>SSGLNDIFEAQKIEWHEGSAGGSGGSGRSSLDNIEMAYARQIYIYNEKIVNGHLQPNLVDLCASVAELDDKSISDMWTMVKQMTDVLLTPATDALKNRSSVEVRMEFVRQALAYLEQSYKNYTLVTVFGNLHQAQLGGVPGTYQLVRSFLNIKLPAPLPGLQDGEVEGHPVWALIYYCMRCGDLLAASQVVNRAQHQLGEFKTWFQEYMNSKDRRLSPATENKLRLHYRRALRNNTDPYKRAVYCIIGRCDVTDNQSEVADKTEDYLWLKLNQVCFDDDGTSSPQDRLTLSQFQKQLLEDYGESHFTVNQQPFLYFQVLFLTAQFEAAVAFLFRMERLRCHAVHVALVLFELKLLLKSSGQSAQLLSHEPGDPPCLRRLNFVRLLMLYTRKFESTDPREALQYFYFLRDEKDSQGENMFLRCVSELVIESREFDMILGKLENDGSRKPGVIDKFTSDTKPIINKVASVAENKGLFEEAAKLYDLAKNADKVLELMNKLLSPVVPQISAPQSNKERLKNMALSIAERYRAQGISANKFVDSTFYLLLDLITFFDEYHSGHIDRAFDIIERLKLVPLNQESVEERVAAFRNFS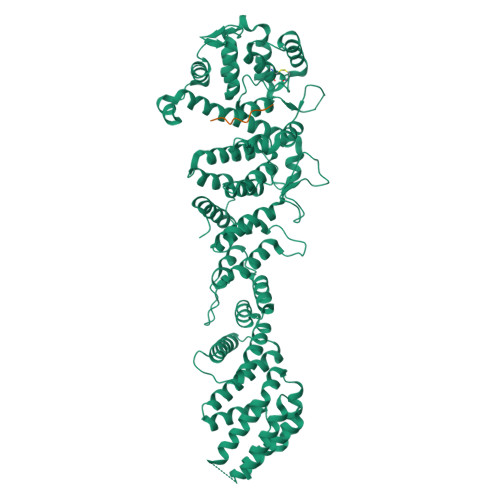DEIRHNLSEVLLATMNILFTQFKRLKGTSPSSSSRPQRVIEDRDSQLRSQARTLITFAGMIPYRTSGDTNARLVQMEVLMN[2x];>SDKSGAPPVRSIYDDISSPGLGSTPLTSRRQPNISVMQSPLVGVTSTPGTGQSMFSPASIGQPRKTTL[2x]>[4x]XXXXXXXXXXXXXXXXXAGKSLPWWAVGASLIAANISAEQFIGMSGSGYSIGLAIASYEWMSAITLIIVGKYFLPIFIEKGIYTIPEFVEKRFNKKLKTILAVFWISLYIFVNLTSVLYLGGLALETILGIPLMYSILGLALFALVYSIYGGLSAVVWTDVIQVFFLVLGGFMTTYMAVSFIGGTDGWFAGVSKMVDAAPGHFEMILDQSNPQYMNLPGIAVLIGGLWVANLYYWGFNQYIIQRTLAAKSVSEAQKGIVFAAFLKLIVPFLVVLPGIAAYVITSDPQL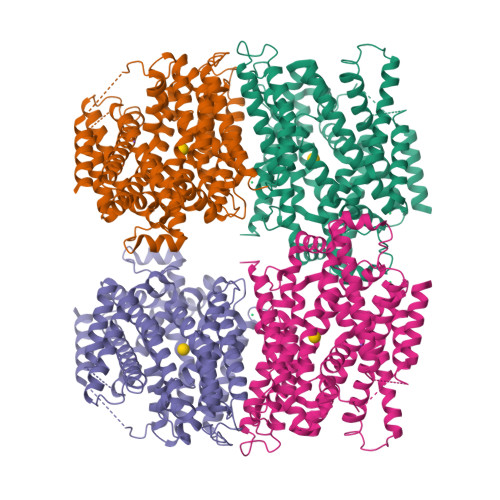MASLGDIAATNLPSAANADKAYPWLTQFLPVGVKGVVFAALAAAIVSSLASMLNSTATIFTMDIYKEYISPDSGDHKLVNVGRTAAVVALIIACLIAPMLGGIGQAFQYIQEYTGLVSPGILAVFLLGLFWKKTTSKGAIIGVVASIPFALFLKFMPLSMPFMDQMLYTLLFTMVVIAFTSLSTSINDDDPKGISVTSSMFVTDRSFNIAAYGIMIVLAVLYTLFWVLYKSGGSPGHHHHHH>GSHMASGPGFDFAQAIMKKNT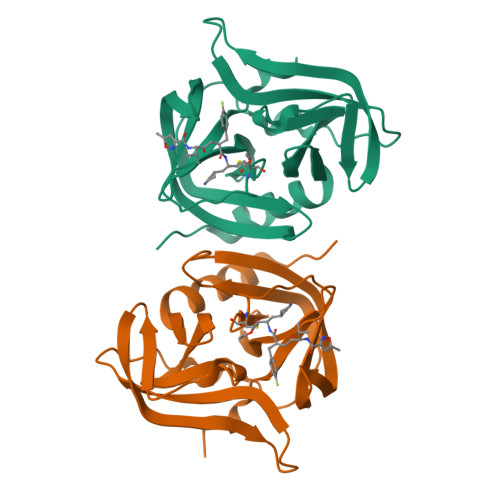VIARTEKGEFTMLGVYDRVAVIPTHASVGETIYINDVETKVLDACALRDLTDTNLEITIVKLDRNQKFRDIRHFLPRYEDDYNDAVLSVHTSKFPNMYIPVGQVTNYGFLNLGGTPTHRILMYNFPTRAGQCGGVVTTTGKVIGIHVGGNGAQGFAAMLLHSYFSDTQ[2x]>[2x]MAPLRTKAVEVLQRNSRGAFTVPAHGLYPYQWLWDSAFIALGWTQVDWERAWQELLCL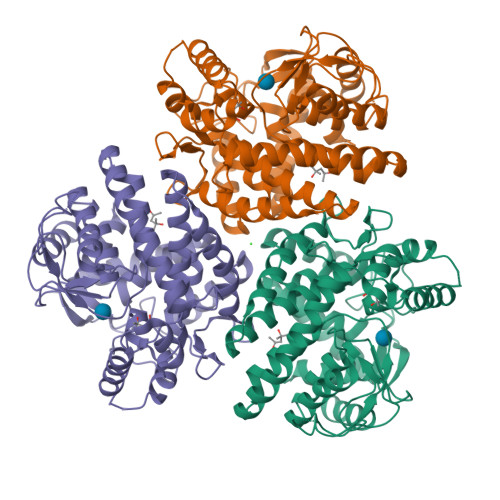FDYGQGPDGMLPHIVFHEQSRDYFPGPDVWGREARAQPATSGITQPPVVATVVRYLYEKDPDRDRARERARYLFPKLLAFHRWLYHARDPYRTGLVVIVHPWESGMDNSPAWDKPLSRVPVENLPPYERRDVKHVNPEERPRKEDYDRYLSLLYLFRRLEYDPREIYRQSPFKVVDVGFNAILQRANRDLYALAVLLQEDPYEIEEWIVRGEVGLEALWDREAGFYFSWDLVAGEPIAVKTSAGFLPLFAGTPHQGRASLLAQEAERWGEKARYLLPSVDPTSPFFEPGRYWRGPVWINVNWMVAEGFRDYGFAALAARLKADALALMEREGFREYYDPLTGQGRGGEGFSWSAALALFWTR If the HK incorporates a REC domain (REC-1) is denoted as hybrid histidine kinase (hHK), and the first His-Asp phosphotransfer event occurs in the same polypeptide chain. Then, HPt protein containing a phosphorylatable His shuffles the phosphoryl group from the phosphorylatable Asp in the REC-1 domain to the phosphorylatable Asp in the REC domain of an RR (REC-2) in two more phosphotransfer steps. In fungi, the HPt accepts the phosphoryl group from REC-1 domains of various hHKs upstream of the signaling pathway and forwards it downstream to REC-2 domains present in at least two conserved RRs, Ssk1 and Skn7. Also, we have obtained the crystal structures of Ct_HPt alone and in complex with REChHK6 bound to the phosphomimetic BeF3−, as well as the crystal structures of REChHK3 and RECCa_Sln1.

We obtained the structure of REChHK3, which contained one molecule in the AU, and we superposed it into REChHK6. Both structures demonstrated overall structural similarity (rmsd value of 1.4 Å for 116 residues aligned), although, α3 and loop α3–β4 were longer in REChHK3. In REChHK3 the Mg2+ ion was stabilized in the active center by interactions with the phosphorylatable D1149, residue D1106 in loop β1–α1, the main chain carbonyl oxygen of Q1151 in loop β3–α3 and two water molecules. Also, the conformation of loop β4–α4 seemed highly mobile with scarce electron density, as observed in REChHK6, and the conformation between both REC-1 domains was different affecting to the spatial position of α4. Meanwhile, a closer inspection of the active center for REChHK3 allowed us to observe that the C-terminal of the highly conserved β4, containing the motif LTA comprised by the conserved Thr (T1183), formed a hydrogen bond (distance ~ 3 Å) with the C-terminal of β3. Specifically, this bond involved the main chain carbonyl oxygen (O) of Leu in β4 (L1182) and the main chain nitrogen (N) of the residue after the phosphorylatable D1149 (Asp + 1) in β3 (OLeu-NAsp+1 distance). Superposed REChHK3 in the complex revealed close contacts with Ct_HPt just for two residues located in α1 which had flexible long side chains (R1112 and K1161); thus, recognition of REC-1 domains seems to involve subtle conformational changes. The absence of the Leu-Thr switch was observed in the structures of REChHK3 and RECCal_Sln1 which were found bound just to Mg2+ion, although we added phosphomimetic in our crystallization mixture. Meanwhile, REChHK3 showed a monomeric species and a small amount of oligomer that we could assign to a trimer, detected in the crystal by the PISA server (buried area of 3935.6 Å2 and a ΔGdiss of 38.9 kcal/mol indicating stability), which shifted to monomer in the presence of PAM.

> GPGENRATPSLADNTRSFEILLAEDNAVNQRLAVKILEKYHHVVTVVGNGEEAVEAVKRKKFDVILMDVQMPVMGGFEATAKIREYEASLPTPQRTPIIALTAHAMMGDREKCLEAQMDEYLSKPLQQANLIQTILKCA> GSSHHHHHHLEVLFQGPVNALVSHLLVVEPEKLYAMPDPAGPDGHLPAVATLCDLFDREIVVTISWAKSIPGFSSLSLSDQMSVLQSVWMEVLVLGVAQRSLPLQDELAFAEDLVLDEEGARAAGLGELGAALLQLVRRLQALRLEREEYVLLKALALANSDSVHIEDAEAVEQLREALHEALLEYEAGRAGPGGGAERRRAGRLLLTLPLLRQTAGKVLAH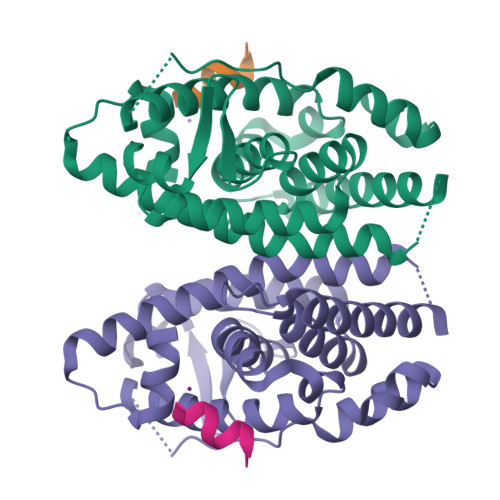FYGVKLEGKVPMHKLFLEMLEAMMD;> RPASELLKYLTT> MHSLQNVIPQQQAHIAELQVYNNKLERDLQNKIGSLTSSIEWYLRSMELDPEIKADIEQQINSIDAINPLHAFDDLESVIRNLISDYDKLFLMF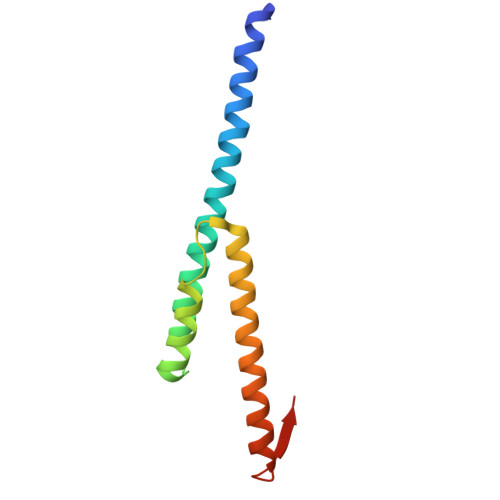KGLIQRSNYQYSFGSE>[4x]AMGSRLYDRRSIFDAVAQSNCQELESLLPFLQRSKKRLTDSEFKDPETGKTCLLKAMLNLHNGQNDTIALLLDVARKTDSLKQFVNASYTDSYYKGQTALHIAIERRNMTLVTLLVENGADVQAAANGDFFKKTKGRPGFYFGELPLSLAACTNQLAIVKFLLQNSWQPADIS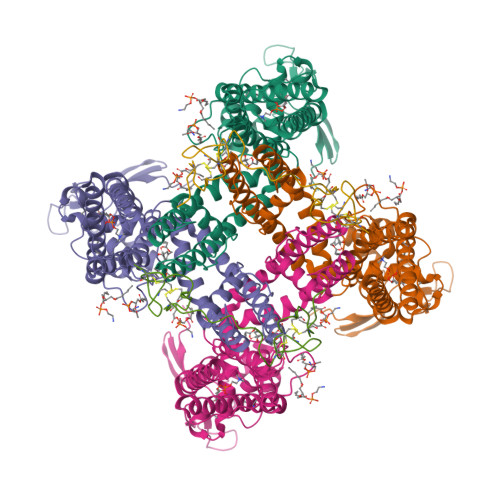ARDSVGNTVLHALVEVADNTVDNTKFVTSMYNEILILGAKLHPTLKLEEITNRKGLTPLALAASSGKIGVLAYILQREIHEPECRHLSRKFTEWAYGPVHSSLYDLSCIDTCEKNSVLEVIAYSSSETPNRHDMLLVEPLNRLLQDKWDRFVKRIFYFNFFVYCLYMIIFTAAAYYRPVEGLPPYKLKNTVGDYFRVTGEILSVSGGVYFFFRGIQYFLQRRPSLKSLFVDSYSEILFFVQSLFMLVSVVLYFSQRKEYVASMVFSLAMGWTNMLYYTRGFQQMGIYAVMIEKMILRDLCRFMFVYLVFLFGFSTAVVTLIEDGKYNSLYSTCLELFKFTIGMGDLEFTENYDFKAVFIILLLAYVILTYILLLNMLIALMGETVNKIAQESKNIWKLQRAITILDTEKSFLKCMRKAFRSGKLLQVGFTPDGKDDYRWCFRVDEVNWTTWNTNVGIINEDPG;>DCAKEGEVCSWGKKCCDLDNFYCPMEFIPHCKKYKPYVPVTTNCAKEGEVCGWGSKCCHGLDCPLAFIPYCEKYR[2x]> MTQSLGIEQYKLSVVSGGKPALNNLSSVTGNK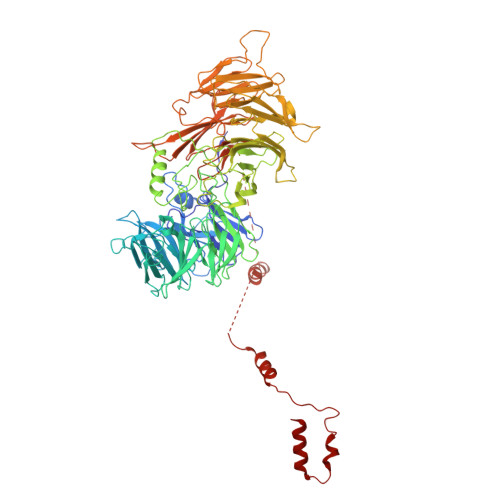NIARLSQDQRNYIIPFNNQIKVYSVETRQCVKTLKFANNSLLSGIFLQEEENNESIVKILLGDITVPQQEDAHLITVFTNNGHVIVLNYKGKLVESPKHFKISLADEKLANVFHSEGNYRILTTFKDPSQKAHNSLQSYRLYALTFDDAKKQFEVAHQAEWHNVILSNISSNGKLLAHMCKDVSTKDHEHKSISVVSLFDDSVNLSFPLGSILSSQTQSLSYNTRYVSSMAIDNMGQQLAVGFASGVISIVSLADLQIRLLKWHIDSVLSLSFSHDGSYLLSGGWEKVMSLWQLETNSQQFLPRLNGIIIDCQVLGPQGNYYSLILQMTENNSNSDYQFLLLNASDLTSKLSINGPLPVFNSTIKHIQQPISAMNTKNSNSITSLNHSKKKQSRKLIKSRRQDFTTNVEINPINKNLYFPHISAVQIFDFYKNEQVNYQYLTSGVNNSMGKVRFELNLQDPIITDLKFTKDGQWMITYEIEYPPNDLLSSKDLTHILKFWTKNDNETNWNLKTKVINPHGISVPITKILPSPRSVNNSQGCLTADNNGGLKFWSFDSHESNWCLKKISLPNFNHFSNSVSLAWSQDGSLIFHGFDDKLQILDFDTFKKFESLENTKTVSEFTLDSEIQTVKLINDTNLIVATRTTLNAINLLRGQVINSFDLYPFVNGVYKNGHMDRLITCDERTGNIALVINQQLTDLDGVPTINYKSRIIIFDSDLSTKLGNFTHHEYISWIGWNYDTDFIFLDIESTLGVVGTXXXXXXXXXXXXXXNDEDEEDIALEFINGEKKDKLVNMNSFTSMFDNIQNVQMDTFFDRVMKVLT> MADRTGIVAGALLPGMPHLLAEHPAPSWSALAGAARDVGARLRRLEPDVVLLLSTQWFTVLGHQFQCDPNPRGEHVDENWYAYDYGLLDYDLRFDVDFTERWADRVQAGGMQARRTRYDGFPIDTGTIVTSALLDPDRRLRWAQVSCNLYADADTLADVGRAGAAAARDAGLRAAVVVVTGMSSG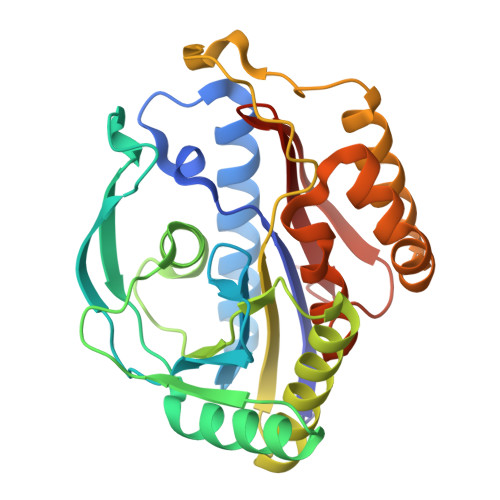LIQQWIEPGQDRIGEPGHDQWNTRVLDLLTAGKVDEVLAVREDFARQAQADSQFRALAFAAGAEATTGPAHLHAYGPIWGTGAAVLSWNLPDHP>MASQPNSSAKKKEEKGKNIQVVVRCRPFNLAERKASAHSIVECDPVRKEVSVRTGGLADKSSRKTYTFDMVFGASTKQIDVYRSVVCPILDEVIMGYNCTIFAYGQTGTGKTFTMEGERSPNEEYTWEEDPLAGIIPRTLHQIFEKLTDNGTEFSVKVSLLEIYNEELFDLLNPSSDVSERLQMFDDPRNKRGVIIKGLEEITVHNKDEVYQILEKGAAKRTTAATLMNAYSSRSHSVFSVTIHMKETTIDGEELVKIG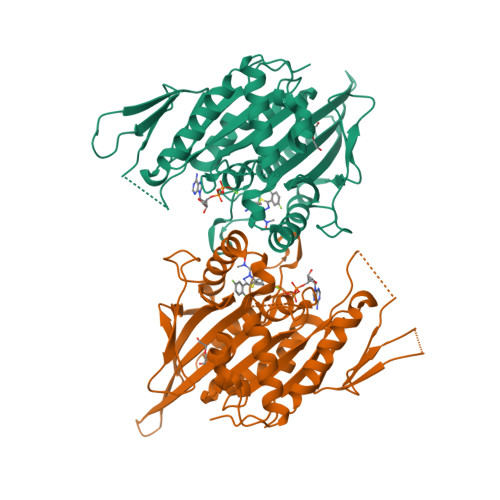KLNLVDLAGSENIGRSGAVDKRAREAGNINQSLLTLGRVITALVERTPHVPYRESKLTRILQDSLGGRTRTSIIATISPASLNLEETLSTLEYAHRAKNILNKPEVNQK[2x]>[2x]MKKLTIGLIGNPNSGKTTLFNQLTGSRQRVGNWAGVTVERKEGQFSTTDHQVTLVDLPGTYSLTTISSQTSLDEQIACHYILSGDADLLINVVDASNLERNLYLTLQLLELGIPCIVALNMLDIAEKQNIRIEIDALSARLGCPVIPLVATD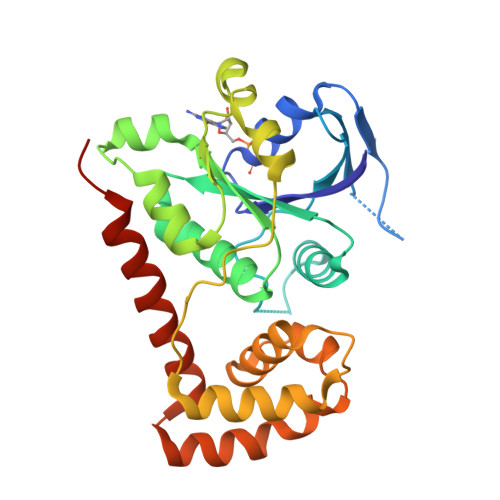TKNVQFVLKLAIDRYKANENVELVHYAQPLLNEADSLAKVMPSDIPLKQRRWLGLQMLEGDIYSRAYAGEASQHLDAALARLRNEMDDPALHIADARYQCIAAICDVVSNTLTAEPSRF> NASSVLASSPKKPVSSYLRFSKEQLPIFKAQNPDAKTTELIRRIAQRWRELPDSKKKIYQDAYRAEWQVYKEEISRFKEQLTPSQIMSLEKEIMDKHLKRKAMTKKKELTLLG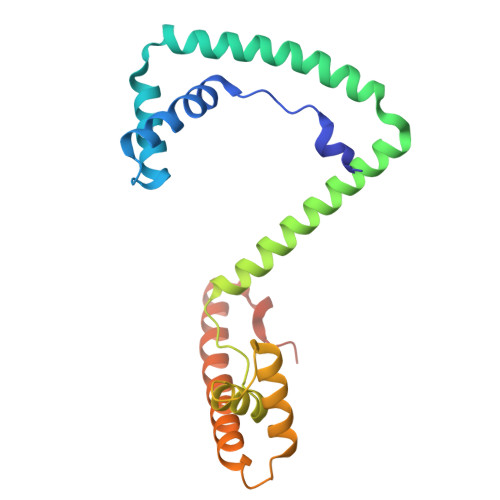KPKRPRSAYNVYVAERFQEAKGDSPQEKLKTVKENWKNLSDSEKELYIQHAKEDETRYHNEMKSWEEQMIEVGRKDLLRRTIKKQRKYGAEE>VSLQEFLKTEPDGTLEVVAEQYNTTLLEVVRNLPSSTVVPGDKFDTVWDTVCEWGNVTTLV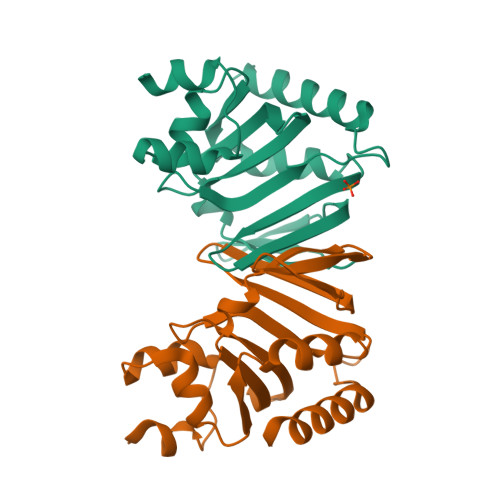HTADVILEFSGELPSGFHRHGYFNLRGKHGMSGHIKAENCTHIALIERKFMGMDTASILFFNKEGSAMLKIFLGRDDHRQLLSEQVSAFHTLAASLKEH[4x]> FASLAPR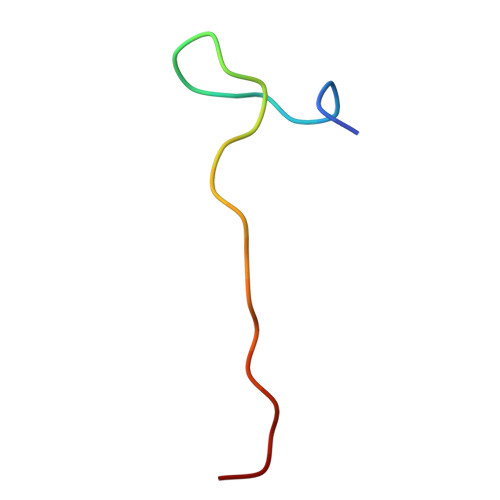HGSRPFMGNWQDIGTSN>MASFEDTLKATIKSNTKQDIKILKIQNLQSSPDVKLVLIAVGNMQVPIFASKDGKLVMGVSNVFFAHKSEDMGAVGSLIKQTQSESKPDKAILDTLFKKIPQDEYIILRSPNKNAKKITYIVSDPNCPSCQKELNNIQERLKDSDVYMLLVGFVGEDSPIKSSMLR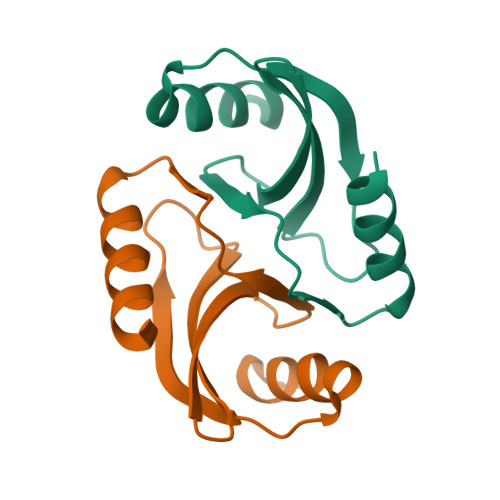DRLLDVKDDKEKLKILREVYTPKSKVPTSYINIDIKDTMKINQKVIDAGIKSVPFVYERNKLEHHHHHHH[2x]>MCLAVPGKVIEVNGPVAVVDFGGVKREVRLDLMPD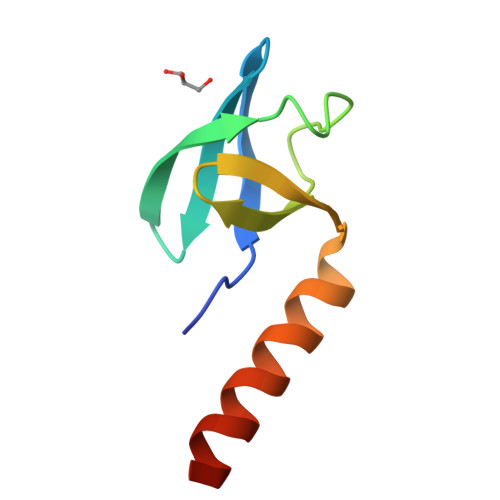TKPGDWVIVHTGFAIEKLDEKKAMEILEAWAEVEKAMEGF[3x]> YS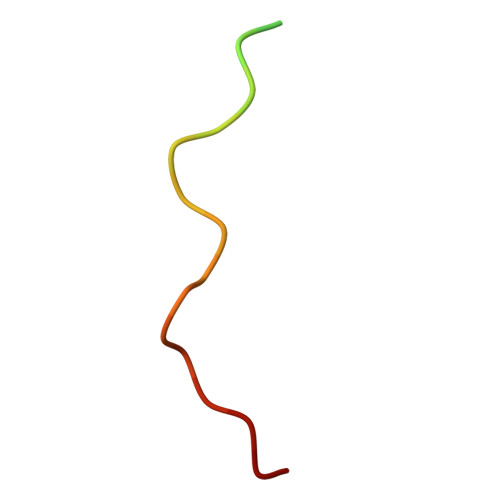NQQSGYGKVSRRGGHQNSYKPY> VLSSQNKKAIEELGNLIKANAEAWGADALARLFELHPQTKTYFSKFSGFEACNEQVKKH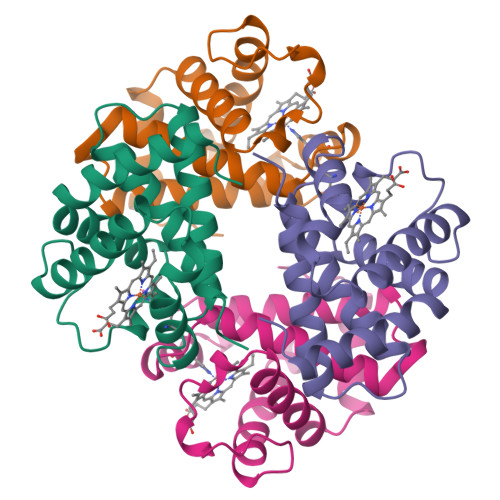GKRVMNALADATHHLDNLHLHLEDLARKHGENLLVDPHNFHLFADCIVVTLAVNLQAFTPVTHCAVDKFLELVAYELSSCYR;> VKLSEDQEHYIKGVWKDVDHKQITAKALERVFVVYPWTTRLFSKLQGLFSANDIGVQQHADKVQRALGEAIDDLKKVEINFQNLSGKHQEIGVDTQNFKLLGQTFMVELALHYKKTFRPKEHAAAYKFFRLVAEALSSNYH2-[(thiophen-2-ylmethyl)amino]-1,7-dihydro-8H-imidazo[4,5-g]quinazolin-8-one | C14 H11 N5 O S | 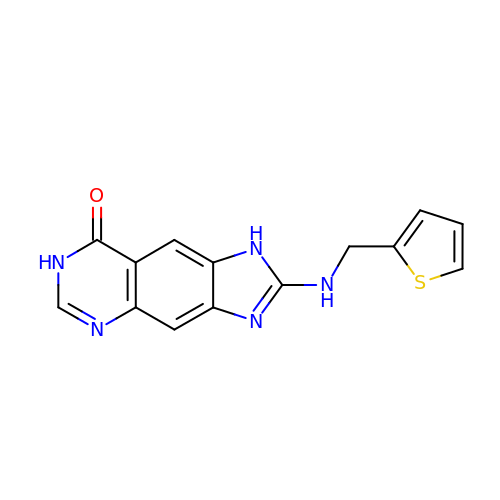FVWYYSMTACIDCC-UHFFFAOYSA-N>[6x]MRENNSGEKTRVLVVGGTGTMGRRIVRACLAEGHETYVLQQPETRVDIEKVQLLYSYKRLGARLIEASFSDHQSLVSAVKQVDIVVAAMSGVHFRSHSILVQLKLVEAIKEAGNIKRFLPSEFGMDPSRMGHAMPPGRETFDQKLEVRNAIEAAGIPHTYVVGACFAAYFAGNLSQMGTLIPPKKKVNIYGDGNVKVVYVDEDDIAEYTAK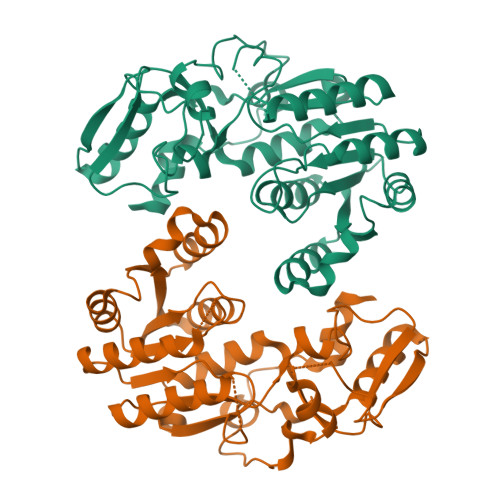TLDDPRTINKTVYVRPTENVLTQMELVQIWEKLTGKELEKTNISANDFLADIEDKEIPHQAGLGHFYHIFYEGCLTDHEVGDDEEASKLYPDVKYTRMDEYLKIFL> ANFENFIGATEGFSEIAYQFTSHILTLGYAVMLAGLLYFILTIKNVDKKFQMSNILSAVVMVSAFLLLYAQAQNWTSSFTFNEEVGRYFLDPSGDLFNNGYRYLNWLIDVPMLLFQILFVVSLTTSKFSSVRNQFWFSGAMMIITGYIGQFYEVSNLTAFLVWGAISSAFFFHILWVMKKVINEGKEGISPAGQKILSNIWILFLISWTLYPGAYLMPYLTGVDGFLYSEDGVMARQLVYTIADVSSKVIYGVLLGNLAITLSKN

Here, we describe a multi-reservoir, high viscosity extruder as a step towards automation of sample delivery at XFELs. After commissioning the device with lysozyme crystals, we collected time-resolved data using crystals of a membrane-bound, light-driven sodium pump. Static data were also collected from the soluble protein tubulin that was soaked with a series of small molecule drugs. In two commissioning beamtimes at the SwissFEL Alvra endstation, we validated the general performance of the multi-reservoir extruder and determined 13 structures overall.

Second, we utilise the device in a time-resolved serial femtosecond crystallography (TR-SFX) experiment by collecting structural snapshots of the light-driven sodium pump Krokinobacter eikastus rhodopsin 2 (KR2).>[2x]MSMAEMLRRDEGLRLKVYWDTEGYPTIGIGHLIMKQPVRDMAQINKVLSKQVGREITGNPGSITMEEATTLFERDLADMQRDIKSHSKVGPVWQAVNRSRQMALENMAFQMGVGGVAKFNTMLTAMLAGDWEKAYKAGRDSLWYQQTKGRASRVTMIILTGNLESYGVELEHHHHHH;>MKKFIFATIFALASCAAQPAMAGYDKDLCEWSMTADQTEVETQIEADIMNIVKRDRPEMKAEVQKQLKSGGVMQYNYVLYCDKNFNNKNIIAEVVGELEHHHHHH[2x]

One of the T4 early gene products produced immediately following the genome injection is gp61.3, also known as Spackle. Spackle, along with another T4 gene product Imm, confers the infected host E. coli with resistance against secondary phage infections—a phenomenon known as “superinfection exclusion”. Our results show that T4 Spackle forms a stoichiometric complex with the lysozyme domain of gp5 and potently inhibits its enzymatic activity, whereas Spackle does not appreciably inhibit the cytoplasmic T4 lysozyme (endolysin, gpe) responsible for cell lysis at the final step of the phage lytic cycle. Crystal structure of the Spackle–gp5 complex shows that the binding of Spackle induces an allosteric conformational change in the gp5 lysozyme active site and partially blocks its oligosaccharide-binding cleft.

To that end, we co-crystallized Spackle and gp5 lysozyme and determined the crystal structure of the complex by molecular replacement phasing. Two crystal forms were obtained, in monoclinic and orthorhombic lattice systems, for which the structures were refined to 1.78 and 1.92 Å resolution, respectively. The monoclinic crystal contained two Spackle–gp5 lysozyme complexes in the asymmetric unit, whereas the orthorhombic crystal contained one complex in the asymmetric unit. In addition, we observed several 4-(2-hydroxyethyl)-1-piperazineethanesulfonic acid (HEPES) molecules bound on the lysozyme surface, including one occupying the oligosaccharide-binding cleft (C-site)20 and another in the peptide-binding groove in the monoclinic crystal structure. The protein structures of the three crystallographically independent complexes were essentially identical to each other, with pairwise backbone room mean square deviations within 0.5 Å. Spackle engages a highly positively charged horseshoe-shaped surface around the deep substrate-binding cleft, spanning both the N and C-terminal lobes of lysozyme. For instance, the main chains of Trp192 and Leu186 from gp5 lysozyme make bidentate hydrogen bonds with the side chain carboxamide moieties of Gln37 and Asn76 from Spackle, respectively; the main-chain carbonyl groups of Ser32, Met33, Thr34, and Ala35 from Spackle at the C-terminus of α1 helix accept a cluster of hydrogen bonds from gp5 lysozyme. Although Spackle binds over and partially blocks a distal site (E/F-site)21 in the substrate-binding cleft of lysozyme, it does not block the enzyme active site or interact directly with the catalytic residues (Glu184 and Asp193). Superposition of Spackle and gp5 lysozyme structures in the complex with their respective unbound state structures shows conformational changes for both proteins upon binding. The conformational change displaces the lysozyme catalytic residues (Glu184 and Asp193), both of which are in the N-terminal lobe, with respect to the oligosaccharide-binding sites.> NKI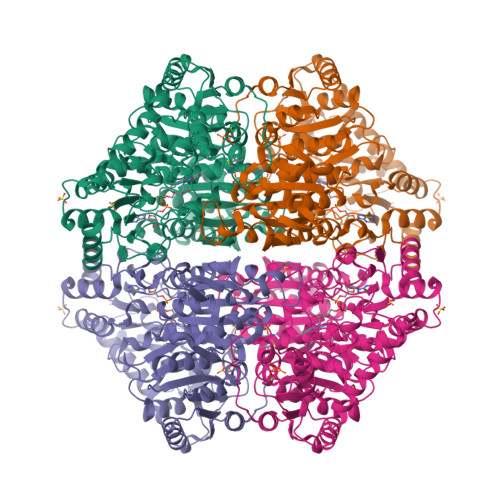NIGLAVMKILESWGADTIYGIPSGTLSSLMDAMGEEENNVKFLQVKHEEVGAMAAVMQSKFGGNLGVTVGSGGPGASHLINGLYDAAMDNIPVVAILGSRPQRELNMDAFQELNQNPMYDHIAVYNRRVAYAEQLPKLVDEAARMAIAKRGVAVLEVPGDFAKVEIDNDQWYSSANSLRKYAPIAPAAQDIDAAVELLNNSKRPVIYAGIGTMGHGPAVQELARKIKAPVITTGKNFETFEWDFEALTGSTYRVGWKPANETILEADTVLFAGSNFPFSEVEGTFRNVDNFIQIDIDPAMLGKRHHADVAILGDAALAIDEILNKVDAVEESAWWTANLKNIANWREYINMLETKEEGDLQFYQVYNAINNHADEDAIYSIDVGNSTQTSIRHLHMTPKNMWRTSPLFATMGIAIPGGLGAKNTYPDRQVWNIIGDGAFSMTYPDVVTNVRYNMPVINVVFSNTEYAFIKNKYEDTNKNLFGVDFTDVDYAKIAEAQGAKGFTVSRIEDMDRVMAEAVAANKAGHTVVIDCKITQDRPIPVETLKLDSKLYSEDEIKAYKERYEAANLVPFREYLEAEGLESKYIK> QRIYSSIEEIIQQAQASEIGQKKEFYVYGNLVSIQMKNKLYYYRCTCQGKSVLKYHGDSFFCESCQQFINPQVHLMLRAFVQDSTGTIPVMIFDQQSSQLINQIDPSIHVQ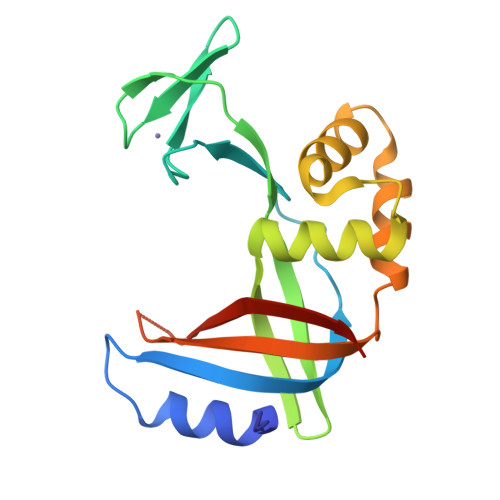EAGQYVKNCIENGQEEIIRQLFSKLDFARFIFEIQFENKEFNNEQEIAYKVLKIEKENIKE>HHHHHHSSGLVPRGSHMETESLPWREYLERIGYQGLLNNSLECLRELYTAHLRSVPYEMLDSFDGTPPVLGHAESFAKLVHRRRGGNCLESTPLFGEFLRQAGFEVRLVPAQIWKVSGEWWDAWDHLLLIVTVDGEDWLLDVGFLMLTFAEPLKVAEGPQEQSGWRFRVAEEEGFPTVSHQGPDGTWTAVYRYRDEPQQRADYEWIIDFHKSAEDSPLVGTLLCS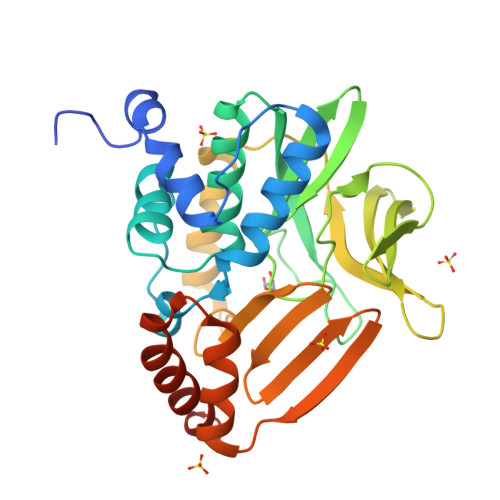RNVPDGKLIMIGENLLHARNGRVSAEFIETTSRAEELLRVIFAGHEHMVESAVRTWEKARADRSTRRSLVYRKAEQ[2x]3-{[(pyridin-2-yl)amino]methyl}phenol | C12 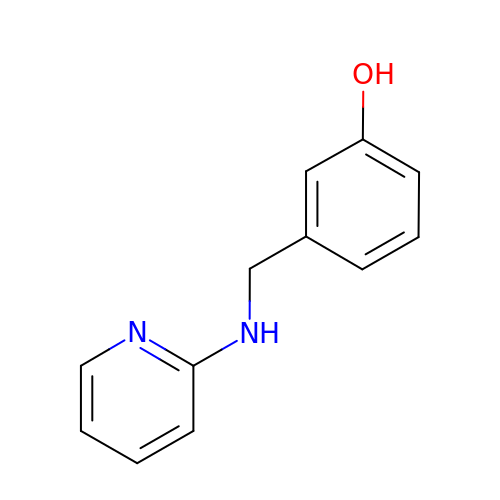H12 N2 O | ZGLJYAOGVJLKLM-UHFFFAOYSA-N Striga hermonthica is a root parasitic plant that infests cereals, decimating yields, particularly in sub‐Saharan Africa. For germination, Striga seeds require host‐released strigolactones that are perceived by the family of HYPOSENSITIVE to LIGHT (ShHTL) receptors. Striga hermonthica has a set of SL receptors, among which ShHTL7 is by far the most sensitive. High‐resolution X‐ray structures reveal that Triton X‐100 specifically plugs the catalytic pocket of ShHTL7.

We determined their structures by molecular replacement, using the ShHTL5 structure as a template 21. Surprisingly, in all crystals, ShHTL7 associated with the 4‐(1,1,3,3‐tetramethylbutyl)‐phenyl hydrocarbon moiety of Triton X‐100 that we used during protein purification (Figs 1A and B and EV1A). Triton bound to the deep active site pocket, formed by a double V‐shaped arrangement of helices α4–α5 and α6–α7. The hydrocarbon moiety of Triton established hydrophobic interactions with Y26 (loop following β2), L124, F134 (β5–α4 loop), M139, T142, L143, L146 (on α4), F150 (α4–α5 loop), L153, T157, L161 (α5), T190, I193, C194 (α7), and M219 (β6–α8 loop; Figs 1C–E and EV2). However, Triton remained at a distance of more than 8 Å from the catalytic serine S95 in the active site. Well‐ordered water molecules filled the space between Triton and the bottom of the active site pocket. The Triton polyethylene head group protruded out of the active site pocket. Five ethylene oxide units were visible in a relatively weak and poorly defined electron density, suggesting weak association of this moiety. The headgroup‐ShHTL7 interactions with the outer rim of the ShHTL7 binding pocket comprised a water‐mediated hydrogen bond (from the oxide of the first unit to the backbone nitrogen of E135) and hydrophobic contacts (between carbons of the first unit and a hydrophobic pocket formed by ShHTL7 V138, M139, and T142, and between carbons of the fourth unit and L160 and I218). In ShHTL7S95C, the sulfhydryl group in C95 was oxidized to a sulfinic acid, as confirmed by mass spectrometry (Fig EV3), causing only a minor rearrangement of the H94 side chain in otherwise identical structures (RMSD of 0.108 Å).

> GPLGSMSSIGLAHNVTILGSGETTVVLGHGYGTDQSVWKLLVPYLVDDYKVLLYDHMGAGTTNPDYFDFDRYSSLEGYSYDLIAILEEFQVSKCIYVGHCMSSMAAAVASIFRPDLFHKLVMISPTPRLINTEEYYGGFEQKVMDETLRSLDENFKSLSLGTAPLLLACDLESAAMQEYCRTLFNMRPDIACCITRMICGLDLRPYLGHVTVPCHIIQSSNDIMVPVAVGEYLRKNLGGPSVVEVMPTEGHLPHLSMPEVTIPVVLRHIRQDITDH> SESQTLDKVYQMKSKPRGYCLIINNHNFAKAREKVPKLHSIRDRNGTHLDAGALTTTFEELHFEIKPHDDCTVEQIYEILKIYQLMDHSNMDCFICCILSHGDKGIIYGT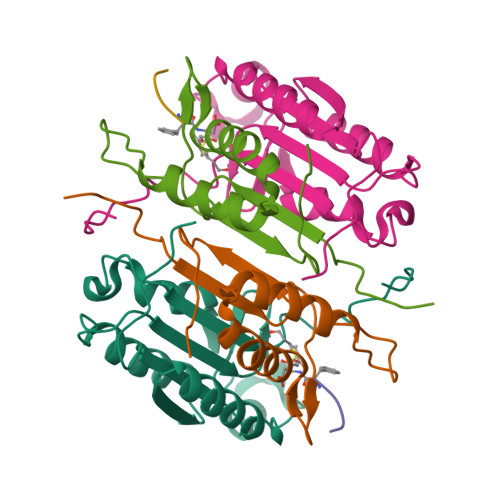DGQEAPIYELTSQFTGLKCPSLAGKPKVFFIQACQGDNYQKGIPVETDSEEQPYLEMD;> LSSPQTRYIPDEADFLLGMATVNNCVSYRNPAEGTWYIQSLCQSLRERCPRGDDILTILTEVNYEVSNKDDKKNMGKQMPQPTFTLRKKLVFPSD>HHHHHHSSGLVPRGSHMQTTTVYSLEDLLPYLKQDNVDVKLAPGTYNVNGFDVGEDRLFSTTPLFLFEGSNSTYDFTDVKLNINTVVLTKFGNNEVNEIQILGNNNVLKNLKLEDIGTTAPSNRAQSIVIDGRDNRIEGFHLTIRGSYPYGYGAAFGKGGGSVINHRKHSGVLIRGLRNHLKDCTIISRSYGHIVFMQAASYPTVEGCYIEGEMRSTDDMLAEEGTGSPADKVDFMTVWGYKLPAGYMMSLQEGGIRAYNAGTTYIDGVEIQRATDNPTVLNCTIKNARTGVTLAHANGTKYVEGCTVLGCENGYSIGSGTVVNCGADAIYGPVFKNTYGSDKGYNADITILPPSDAYYNGHDAVAYIGGSNHNLTFRSEITEIPSNLKIMVSGDLQGLRVLHGSNPSQNNFAGTNIVLRNLTNFPVDLHSDSSNITVTSCDTDNITDNGTNNSIEAIDCDSD[2x]

FdlA from Flavobacterium sp. SA-0082 is an endo-type fucoidan-degrading enzyme that cleaves the sulfated fuco-glucuronomannan (SFGM) through a lytic mechanism. We show that the FdlA-NTD adopts a right-handed parallel β-helix fold, and possesses a substrate binding site composed of a long groove and a unique alkaline pocket. Our structural, biochemical, and enzymological analyses strongly suggest that FdlA-NTD utilizes catalytic residues different from other β-helix polysaccharide lyases, potentially representing a novel polysaccharide lyase family. Here, we report crystal structures and enzymological characterization of wild type (WT) and eight single mutants of the catalytic N-terminal domain (NTD) of FdlA, revealing its unique substrate binding pocket and identifying the key catalytic residues.

We first measured the enzymatic activity of 12 mutants and found that eight of them (D137A, K141A, H176A, F179A, E236A, R240A, Y242A, and Y242F) almost completely abolished their activities, H279A mutant retained approximately 65% of the activity compared with WT, while mutations of Asn243, Arg272, and Tyr322 to Ala only negligibly affect their activities. In the WT structure, both Asp137 and Glu236 form hydrogen bonds with Arg272, while Arg272 participates in the shaping of the alkaline pocket. In both D137A and E236A mutant structures, the side chain of Arg272 switches to the opposite direction compared with that in WT due to the loss of the acidic residue (Arg272 in E236A mutant also exhibits an alternative conformation similar to that in WT), and partially occupies the deep substrate pocket. These results suggest that the steric hindrance of Arg272 in the two mutants may interfere with the substrate fully entering the pocket and hence the correct positioning of the glycosidic O atom, thus resulting in the complete loss of activities of D137A and E236A mutants. We found that the inactive FdlA-NTD mutants exhibited similar Kd values as the wild-type form. These binding assay data clearly demonstrated that while our inactive mutants lost their catalytic activity, they maintained their substrate binding ability.>[2x]SYDYMEGGDIRVRRLFCRTQWYLRIDKR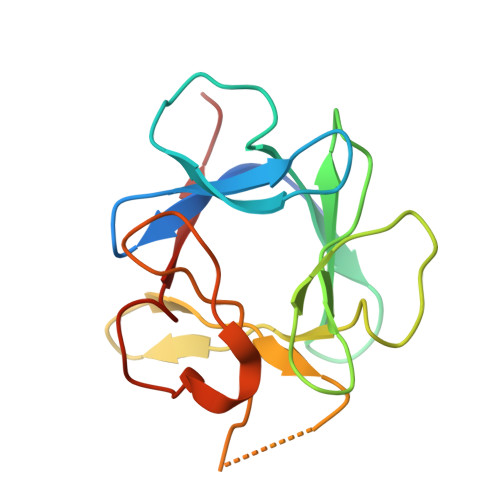GKVKGTQEMRNSYNIMEIRTVAVGIVAIKGVESEYYLAMNKEGKLYAKKECNEDCNFKELILENHYNTYASAKWTHSGGEMFVALNQKGLPVKGKKTKKEQKTAHFLPMAIT> GSARSSSYSGEYGSGGGKRFSHSGNQLDGPITALRVRVNTYYIVGLQVRYGKVWSDYVGGRNGDLEEIFLHPGESVIQVSGKYKWYLKKLVFVTDKGRYLSFGKDSGTSFNAVPLHPNTVLRFISGRSGSLIDAIGLHWDV

ZG16p is a soluble mammalian lectin, the first to be described with a Jacalin-related β-prism-fold. Zymogen granule protein 16 (ZG16p)5 is a 16-kDa soluble protein, originally identified by screening a cDNA expression library of rat pancreas with a polyclonal antibody to purified rat zymogen granule membranes. In conclusion, ZG16p possesses a unique multiple-ligand binding property toward short chain α-manno-oligosaccharides, and sulfated GAG oligosaccharides. The differing carbohydrate-binding modes are attained by a shallow mannose binding pocket and a basic amino acid patch on the protein surface.

Furthermore, two disaccharide-binding modes were observed, enabling the non-reducing or reducing sugar to be accommodated in the binding pocket. O1 of the reducing mannose residue makes a hydrogen bond with the Ser148 O, thus stabilizing the reducing mannose outside the binding pocket.> MIPALIETVIGCLLHDIGKPVQRAALGYRGRHSAIGRAFVKKIWLRDGRNPSEFADEVYEPDIEVFDRRILDAISYHHSSALRTAAENGRLAADAPAYVAYIADNIAAGTDRRKADSDDGQGASTWDSDTPLYSVFNRFGADTANLTFAPEMLDDREPMNIPSARRIEFDKYRYTEIVNKLEAVLVDLECSDTYLASLLNVLEATLSFVPSSTDASEVVDVSLFDHLKLTGALGACIWHYLQATGQSDFKSALFDKQDTFYNEKAFLLTTFDVSGIQDFIYTIHSSGAAKMLRARSFYLEMLTEHLIDELLARVGLSRANLNYSGGGHAYLLLPNTEFARNSLEEFEREANEWLLENFATWLFIATGSVPLAANDLMRRPNESGPQAHDRALRYSGLYRELSEQLSAKKLARYSADQLRELNSSDHDGQKGDRECSVCHTVNRTIKTINDLLLCSLCQALTAASQQIQSESRRFLLISEESSDGLPLPFGATLTFCSESGAKQALQQPQTRRLYAKNKFFAGESLGTGLWVGDYVAQMEFGDYVKRASGIARLGVLRLDVDNLGQAFTHGFMKQGNGKFNTISRTAAFSRMLSLFFRQHINYVLKHPKLRPLTGDDPERSRRATIIYSGGDDVFVVGAWDDVIEFGIELRERFHEFTQGKLTVSAGIGMFPDKYPISVMAREVGDLEGAAKSLPGKNGVALFDPEFTFRWDELLSKVIEEKYRHIADYFRCNEERGMAFIYKLLELLDQRGDRITEARWVYFLMRMRGPTDDTTRFQQFANRLHQWFQDPSDAKQLKTALHLYIYRNRKEESE;>MSVIQDDYVKQAEQVIRGLPKKNGDFELTTTQLRVLLSLTAQLFDEAQLSSDQNLSPALRDKVQYLRVRFVYQAGREKAVRVFVERAGLLDELAQIGDSRDRLLKFCHYMEALVAYKKFLDPKETSKETE[5x];>MITGYAKIEITGTITVVTGLHIGAGDGFSAIGAVDKPVVRDPLTKWPMIPGTSLKGKVRTLLSRQYGADTETFYRKPNDDPAQIRRLFGDTKEYKTGRLVFRDTKLTNKDDLEARGAKTLTEVKFENAINRVTAKANPRQMERVIPGSEFAFSLVYEVSFGTPDEEQKASLPSSDEIIEDFNAIARGLKLLELDYLGGSGTRGYGQVKFSDLKARAAVGTLDRSLLEMLNHELAAV[6x];> MNSRLFRFDVVRTHFGDHGLESSTIGCPADTLYS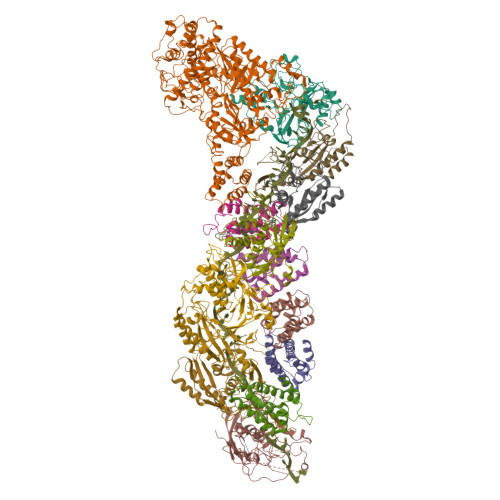ALCVEALRMGGQQLLDELVACSTLRLTDLLPYVGPDYLVPKPLKSVRSDSSSLQKKLAKKIGFLPAAQLGSFLDGTADLDDLAARQTKIGVHAVSAKAAIHNGKKDADPYRVGYFRFEPDAGLWLLATGSESELGLLTRLLKGISALGGERTSGFGAFIPTESEVPAALTPTTAAASLMTLTTSLPTDDELEQALAGATYRLVKRSGFVASATYAETPRRKRDIYKLAAGSVFSRPFQGGILDVSLGGNHPVYSYARPLFLALPESAA;> MSQYLKPFELTLRCLGPVFIGSGEKRTPKEYVASTSMVYFPDMERLYADVAAQGKSESFEEFMMNTGKAQPDERFNEWIAENGVKVSPKNHGGYGVKIGSIVPGRAHRGRDGQMIQEQRQLNDIHSFIKDVLGNPYVPGSSVKGMLRSIYLQSLVHQRTAQPVRVPGHQTREHRQYGERFERKELRKSGRPNTRPQDAVNDLFQAIRVTDSPGLRTSDLLICQKMDVNVHGKPDGLPLFRECLAPGTSISLRVVVDTSPTARGGWPAGERFLETLSDTVAFVNKARYAEYAAKYWDDDPQFGPIVYLGGGAGYRSKTFVTQQDDMAKVLDAQFPKIKHVAKTRDLGVSPLVLKLTKIGDKYYEMGQCELSIRRAE>[2x]MKTFAAYVIIACLSSTALAGSITENTSWNKEFSAEAVNGVFVLCKSSSKSCATNDLARASKEYLPASTFKIPNAIIGLETGVIKNEHQVFKWDGKPRAMKQWERDLTLRGAIQVSAVPVFQQIAREVGEVRMQKYLKKFSYGNQNISGGIDKFWLEGQLRISAVNQVEFLESLYLNKLSASKENQLIVKEALVTEAAPEYLVHSKTGFSGVGTESNPGVAWWVGWVEKETEVYFFAFNMDIDNESKLPLRKSIPTKIMESEGIIGG

Carbapenemases are the main cause of carbapenem resistance in Gram‐negative bacteria. How β‐lactamases with weak carbapenemase activity, such as the OXA‐10‐type class D β‐lactamases, contribute to anti‐bacterial drug resistance is unclear. OXA‐655 is a T26M and V117L OXA‐10 variant, recently identified from hospital wastewater. Here, we have solved crystal structures of OXA‐10 in complex with imipenem (IPM) and ETP, and OXA‐655 in complex with MEM in order to unravel the structure–function relationship and the impact of residue 117 in enzyme catalysis.

In summary, the crystal structures highlight the importance of residue 117 in OXA‐10 variants for carbapenemase activity. This study also illustrates the impact of a single amino acid substitution on the substrate profile of OXA‐10 and the evolutionary potential of new OXA‐10 variants.> MGSMIKTIAFGRYELDTWYHSPYPEEYARLGRLYMCEFCLKYMKSQTILRRHMAKCVWKHPPGDEIYRKGSISVFEVDGKKNKIYCQNLCLLAKLFLDHKTLYYDVEPFLFYVMTEADNTGCHLIGYFSKEKNSFLNYNVSCILTMPQYMRQGYGKMLIDFSYLLSKVEEKVGSPERPLSDLGLISYRSYWKEVLLRYLHNFQ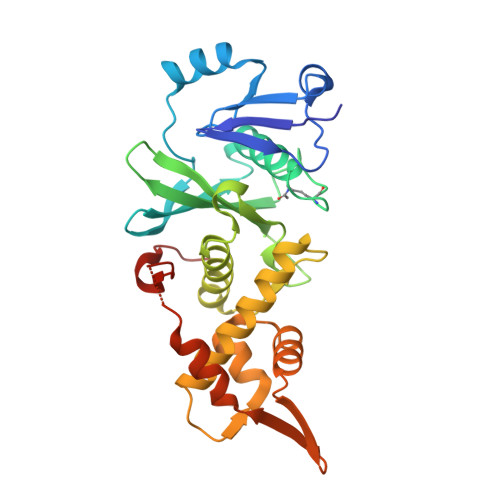GKEISIKEISQETAVNPVDIVSTLQALQMLKYWKGKHLVLKRQDLIDEWIAKEAKRSNSNKTMDPSCLKWTPPKAS>[4x]SNAALLTAKTFSLQFNNKRRVNKPYYPRKALLCYQLTPQNGSTPTRGHLINKKEDHAEIRFINEIKSMGLDETQCYQVTCYLTWSPCPSCAGELVDFIKAHRHLNLRIFASRLYYHWHPNYQEGLLLLCGSQVPVEVMGLPEFTDCWENFVDHKEPPSFNPSEKLKELDKNSQAIKRRLERIKSRSVDVLENGLRSLQLGPVTPSSSIRNSRGGR

APOBEC3 (apolipoprotein B mRNA-editing enzyme, catalytic polypeptide-like, family 3; “A3”) antiviral proteins cause lethal G-to-A hypermutation in retroviruses and retroelements by converting deoxycytosine to deoxyuracil in newly reverse-transcribed single-stranded DNA (ssDNA). A3 proteins are comprised of one (A3H) or two (A3F and A3G) “Z” domains containing Zn-coordinating His and Cys amino acids that, together with a conserved Glu, form the deaminase catalytic center. A3H is an attractive target for biochemical and structural study because the single Z3 domain possesses all three biochemical activities: cytidine deaminase, RNA binding, and Vif binding. RNA binding is a key feature of A3 proteins that is necessary for their encapsidation into virions and for antiviral activity.

Here, we present the 2.24-Å crystal structure of a full-length, natural polymorphic variant of pig-tailed macaque APOBEC3H (pgtA3H) bound to a short RNA duplex. The pgtA3Hζ structure was solved using the anomalous scattering of the native Zn ion at the active site of the enzyme, resulting in a high-quality 2.24-Å structure. A3H has the familiar A3 fold composed of a five-stranded central β-sheet surrounded by six α-helices, and is highly similar to structures of other A3s in the overall fold and in the active site18. Two A3H molecules form a complex with one RNA duplex. The A3H–RNA complex is maintained solely through protein–RNA contacts; there are no direct contacts between A3H protein molecules. Of the nine nucleotides in each strand (nt1–9), seven are base paired (nt3–9) and the two 5′ nucleotides (nt1 and nt2) are unpaired. A sharp kink in the RNA between nt1 and nt2 brings the 5′ nucleotides close to one another and results in stacking of the nt1 bases, which are sandwiched between the phenolic rings of Tyr23 in the two A3H molecules. The RNA kink is stabilized by A3H loop 1 (residues 13–30), which inserts into the narrow major groove of the A-form RNA duplex and includes a unique four-residue insertion (22PYYP25). The unpaired nt2 base protrudes into an A3H “aromatic cage” composed of amino acids from loop 7 (Tyr112, Tyr113, and Trp115) and loop 3 (Trp82). In summary, A3H is selective for RNA through a strong conformational preference for an A-form duplex with seven base pairs, but it lacks sequence specificity.> SRVIVHVDLDCFYAQVEMISNPELKDKPLGVQQKYLVVTCNYEARKLGVKKLMNVRDAKEKCPQLVLVNGEDLTRYREMSYKVTELLEEFSPVVERLGFDENFVDLTEMVEKRLQQLQSDELSAVTVSGHVYNNQSINLLDVLHIRLLVGSQIAAEMREAMYNQLGLTGCAGVASNKLLAKLVSGVFKPNQ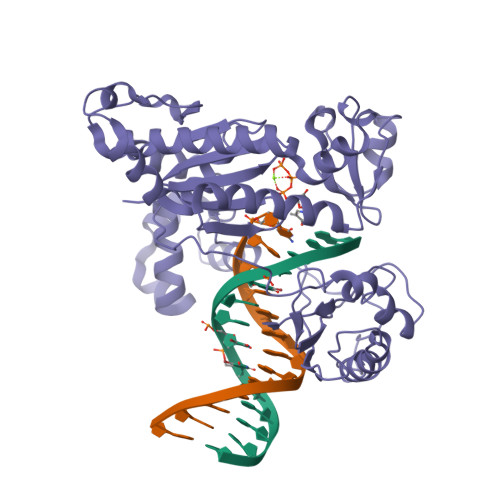QTVLLPESCQHLIHSLNHIKEIPGIGYKTAKCLEALGINSVRDLQTFSPKILEKELGISVAQRIQKLSFGEDNSPVILSGPPQSFSEEDSFKKCSSEVEAKNKIEELLASLLNRVCQDGRKPHTVRLIIRRYSSEKHYGRESRQCPIPSHVIQKLGTGNYDVMTPMVDILMKLFRNMVNVKMPFHLTLLSVCFCNLK> MKVFCGRANPTTGSLEWLEEDEHYDYHQEIARSSYADMLHDKDRNIKYYQGIRAAVSRVKDRGQKALVLDIGTGTGLLSMMAVTAGADFCYAIEVFKPMAEAAVKIVERNGFSDKIKVINKHSTEVTVGPDGDLPCRANILITELFDTELIGEGALPSYEHAHKHLVQEDCEAVPHRATVYAQLVESRRMWSWNKLFPVRVRTSLGEQVIVPPSELERCPGAPSVCDIQLNQVSPADFTVLSDVLPMFSVDFSKQVSSSAACHSRQFVPLASGQAQVVLSWWDIEMDPEGKIKCTMAPFWAQTDPQELQWRDHWMQCVYFLPQEEPVVQGSPRCLVAHHDDYCVWYSLQRTSPDENDSAYQVRPVCDCQAHLLWNRPRFGEINDQDRTDHYAQALRTVLLPGSVCLCVSDGSLLSMLAHHLGAEQVF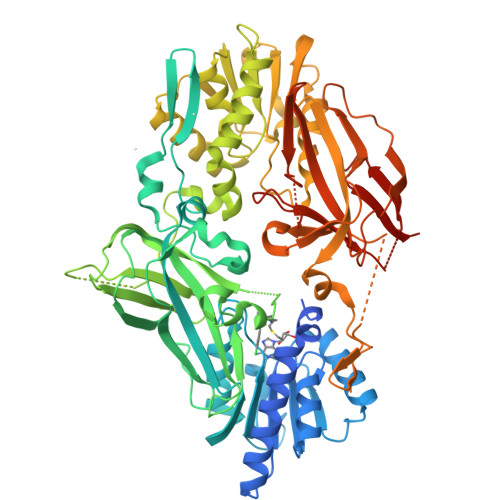TVESSVASYRLMKRIFKVNHLEDKISVINKRPELLTAADLEGKKVSLLLGEPFFTTSLLPWHNLYFWYVRTSVDQHLAPGAVVMPQAASLHAVIVEFRDLWRIRSPCGDCEGFDVHIMDDMIKHSLDFRESREAEPHPLWEYPCRSLSKPQEILTFDFQQPIPQQPMQSKGTMELTRPGKSHGAVLWMEYQLTPDSTISTGLINPAEDKGDCCWNPHCKQAVYFLSTTLDLRVPLNGPRSVSYVVEFHPLTGDITMEFRLADTLS[4-(5-chloranyl-[1,3]oxazolo[4,5-b]pyridin-2-yl)piperazin-1-yl]-[2-[4-(1-cyclobutylcyclopropyl)pyridin-3-yl]-1,3-benzoxazol-6-yl]methanone 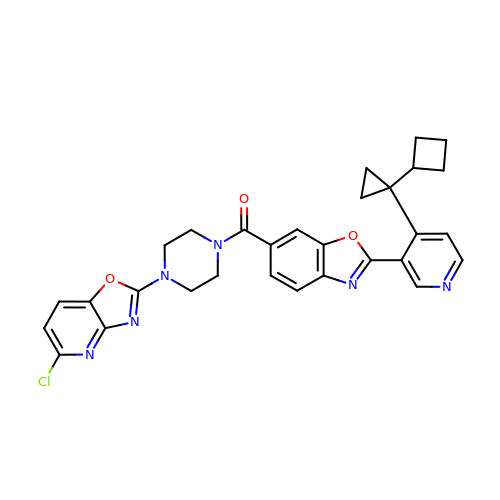| C30 H27 Cl N6 O3 | MXJHPFWCVCDTIM-UHFFFAOYSA-N> SNADSGQSLVPVYIYSPEYVSMCDSLAKIPKRASMVHSLIEAYALHKQMRIVKPKVASMEEMATFHTDAYLQHLQKVSQEGDDDHPDSIEYGLGYDCPATEGIFDYAAAIGGATITAAQCLIDGMCKVAINWSGGWHHAKKDEASGFCYLNDAVLGILRLRRKFERILYVDLDLHHGDGVEDAFSFTSKVMTVSLHKFSPGFFPGTGDVSDVGLGKGRYYSVNVPIQDGIQDEKYYQICESVLKEVYQAFNPKAVVLQLGADTIAGDPMCSFNMTPVGIGKCLKYILQWQLA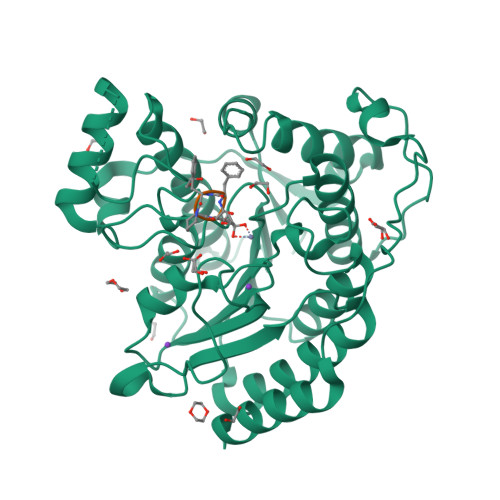TLILGGGGYNLANTARCWTYLTGVILGKTLSSEIPDHEFFTAYGPDYVLEITPSCRPDRNEPHRIQQILNYIKGNLKHVV We have previously studied an endogenous protein, called LCN2, also known as Neutrophil Gelatinase Associated Lipocalin (NGAL) or Siderocalin (Scn), which has several characteristics useful for the safe excretion of iron. Second, LCN2 captures catecholates, which in turn bind iron; these are produced by Gram negative bacteria, such as the siderophore Enterochelin (Ent), and potentially by mammals, such as the catechol metabolites of amino acids and dietary polyphenols. The ligation of Ent:Fe3+ by LCN2 is a critical step in bacteriostasis because sequestration of Ent:Fe3+ reduces iron transport to bacteria and limits their growth. Fifth, the kidney captures the majority of circulating LCN2 (50–70%) via filtration followed by reabsorption from the lumen of the proximal tubule, whereupon it is degraded.

Hence, to identify residues required for megalin binding, we mutated 18 positively charged amino acids on the surface of LCN2, based on information from its crystal structure (K15, 46, 50, 59, 62, 73, 74, 75, 98, 118, 142, 149, 157; H165; and R43, 72, 130, 140). We found 13 LCN2 mutants that could load with Ent:55Fe and then could traffic through the kidney into the urine, particularly K3 (19% of input). To define the structural basis for iron trafficking by K3, we solved its crystal structure. Views of the molecular surfaces of LCN2 (top) and K3 (bottom) coloured according to electrostatic potentials, showed the large effect on the chemical character of LCN2 by the resurfacing mutations. Nonetheless, superposition of native and K3 structures demonstrated a high degree of overall structural conservation, including complete conservation of the ligand-binding site. In other words, neither the fold nor the ligand-binding site of LCN2 were affected by the mutation of surface residues, allowing K3 and K3Cys to efficiently traffic Ent:iron. The addition of native or K3, however completely blocked the Ent- or catechol-mediated conversion of Fe+3 to Fe+2 (P<0.05±LCN2 with either Ent or catechol:iron, Student's t-test; n=3 each) and the subsequent oxidation of HPF to fluorescein (P<10−7, Student's t-test, n=3, across all points). In sum, biochemical, cellular and animal data, suggested the hypothesis that K3 and K3Cys bypassed the proximal tubule as a result of a failure to recognize megalin. Fortunately, K3 maintains almost all structural and functional features of the native protein permitting iron transport.

>[2x]QDSTSDLIPAPPLSSVPLQQNFQDNQFQGKWYVVGLAGNAILREDEDPQKMYATIYELKEDKSYNVTSVLFRDDGCDYWIRTFVPGCQPGEFTLGNIQSYPGLTSYLVRVVSTNYNQFAMVFFKKVSQNQEYFKITLYGRTKELTSELQENFIRFSKSLGLPENNIVFPVPIDQCIDG> EIKFEF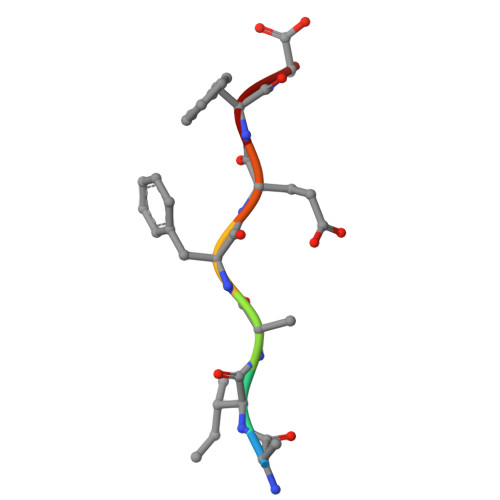D> SEAEARPTNFIRQIIDEDLASGKHTTVHTRFPPEPNGYLHIGHAKSICLNFGIAQD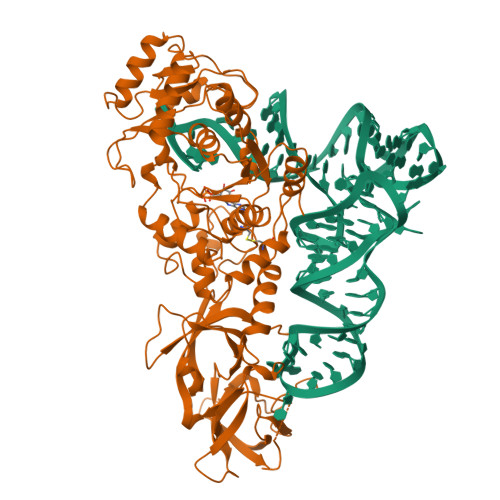YKGQCNLRFDDTNPVKEDIEYVESIKNDVEWLGFHWSGNVRYSSDYFDQLHAYAIELINKGLAYVDELTPEQIREYRGTLTQPGKNSPYRDRSVEENLALFEKMRAGGFEEGKACLRAKIDMASPFIVMRDPVLYRIKFAEHHQTGNKWCIYPMYDFTHCISDALEGITHSLCTLEFQGNRRLYDWVLDNITIPVHPRQYEFSRLNLEYTVMSKRKLNLLVTDKHVEGWDDPRMPTISGLRRRGYTAASIREFCKRIGVTKQDNTIEMASLESCIREDLNENAPRAMAVIDPVKLVIENYQGEGEMVTMPNHPNKPEMGSRQVPFSGEIWIDRADFREEANKQYKRLVLGKEVRLRNAYVIKAERVEKDAEGNITTIFCTYDADTLSKDPADGRKVKGVIHWVSAAHALPVEIRLYDRLFSVPNPGAADDFLSVINPESLVIKQGFAEPSLKDAVAGKAFQFEREGYFCLDSRHSTAEKPVFNRTVGLRDTWAKVGE(4R)-3-[(2S,3S)-3-[[(2R)-2-[2-(4-hydroxyphenyl)ethanoylamino]-3-methylsulfanyl-propanoyl]amino]-2-oxidanyl-4-phenyl-butanoyl]-5,5-dimethyl-N-[(1S,2R)-2-oxidanyl-2,3-dihydro-1H-inden-1-yl]-1,3-thiazolidine-4-carboxamide | C37 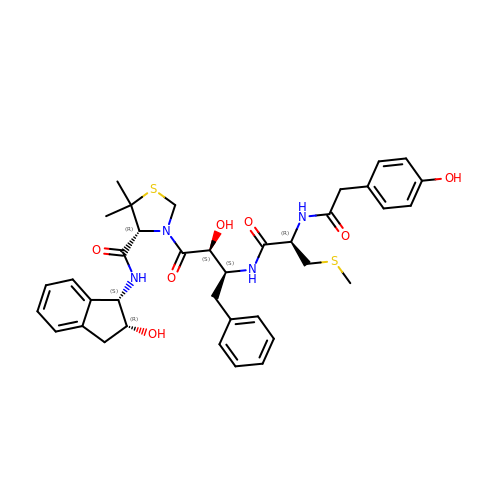H44 N4 O7 S2 | OONNUXMESNYHOP-ACUZRORGSA-N>QDDLTISSLAKGETTKAAFNQMVQGHK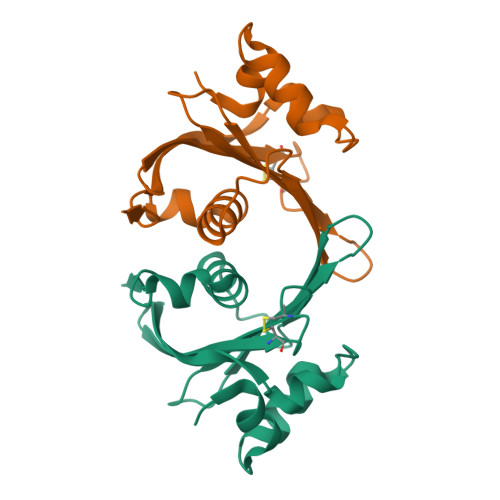LPAWVMKGGTYTPAQTVTLGDETYQVMSACKPHDCGSQRIAVMWSEKSNQMTGLFSTIDEKTSQEKLTWLNVNDALSIDGKTVLFAALTGSLENHPDGFNFRSHHHHHH[3x]>[2x]MEKFVLSLDEGTTSARAIIFDRESNIHGIGQYEFPQHYPRPGWVEHNPEEIWDAQLRAIKDAIQSARIEPNQIAAIGVTNQRETTLVWDKDGKPLYNAIVWQCRRTAEMVEEIKREYGTMIKEKTGLVPDAYFSASKLKWLLDNVPGLREKAEKGEVMFGTVDTFLIYRLTGEHVTDYSNASRTMLFNIKK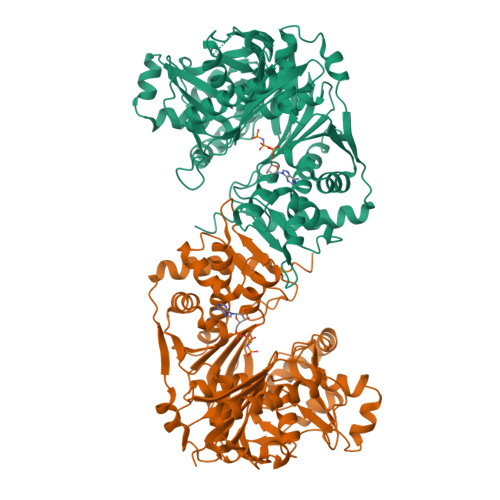LDWDDELLELFDIPESVLPEVRESSEVYGYTKKELLGAEIPVSGDAGDQQAALFGQAAFEAGMVKATYGTGSFILVNTDKMVLYSDNLLTTIAWGLNGRVSYALEGSIFVTGAAVQWLRDGIKIIKHASETEELATKLESNEGVYFVPAFVGLGAPYWDQFARGIIIGITRGTGREHLARATLEAIAYLTRDVVDEMEKLVQIKELRVDGGATANDFLMQFQADILNRKVIRPVVKETTALGAAYLAGLAVDYWADTREIAELWKAERIFEPKMDEKTRERLYKGWKEAVKRAMGWAKVVDSAKSN> GHQPVAEERLSALLLNSSEVN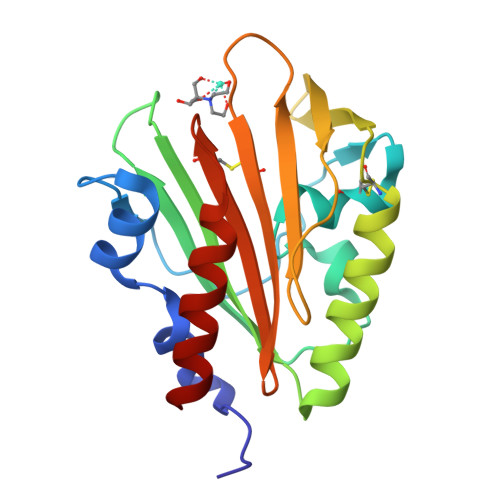AVMGSSSMQPGKPITSMDSSPVTVSLPDCQGALYTSQDPVYAGTGYTAINGLISSEPGDNYEHWVNQAVVAFPTADKARAFVQTSADKWKNCAGKTVTVTNKAKTYRWTFADVKGSPPTITVIDTQEGAEGWECQRAMSVANNVVVDVNACGYQITNQAGQIAAKIVDKVNKE>NPREEILDASAELFTRQGFATTSTHQIADAVGIRQASLYYHFPSKTEIFLTLLKSTVEPSTVLAEDLSTLDAGPEMRLWAIVASEVRLLLSTKWNVGRLYQLPIVGSEEFAEYHSQREALTNVFRDLATEIVGDDPRAELPFHITM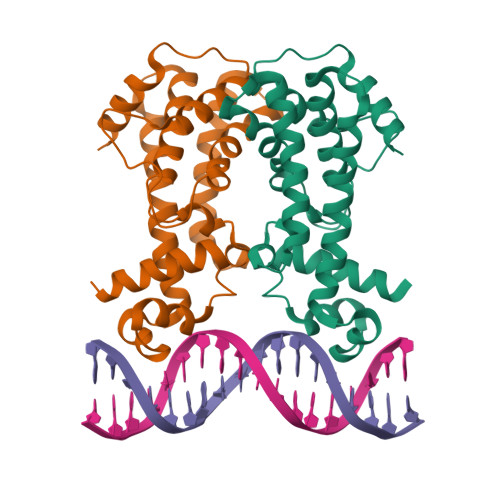SVIEMRRNDGKIPSPLSADSLPETAIMLADASLAVLGAPLPADRVEKTLELIKQAD[2x]> MQLV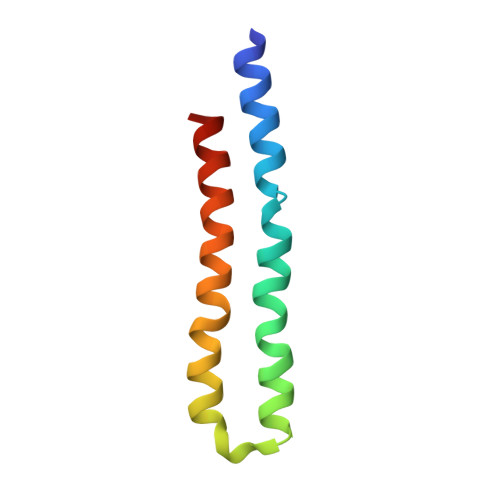LAGKYIGAGLASIGLVGAGIGIAIVFAALINGVSRNPALKGQLFTYSILGFALSEATGLFALMIAFLLLYAV The enzyme, pyranose dehydrogenase (PDH), from the filamentous fungus Coprinopsis cinerea (CcPDH) of the Basidiomycete division, is composed of a catalytic PQQ-dependent domain classified as a member of the novel auxiliary activity family 12 (AA12), an AA8 cytochrome b domain, and a family 1 carbohydrate-binding module (CBM1), as defined by the Carbohydrate-Active Enzymes (CAZy) database. In the catalytic cycle of CcPDH, electrons are transferred from the reduced PQQ in the AA12 domain to heme b in the AA8 domain, which acts as a built-in mediator and transfers electrons to a heterogeneous electron acceptor. Therefore, CcPDH is thought to be involved in the extracellular oxidative degradation of the plant cell wall. Here, we present the crystal structures of the AA12 domain in its apo- and holo-forms and the AA8 domain of this enzyme.

The AA8 domain of CcPDH was determined at a 1.8-Å resolution, and the final model was refined to R and Rfree values of 15.7% and 20.4%, respectively. The asymmetric unit of the AA8 domain crystal contains a single AA8 domain (residues 21 to 215 of the full-length CcPDH) with a single b-type heme, 2 2-methyl-2,4-pentanediol molecules, 1 acetate ion, and 155 water molecules. AA8 proteins fold into an immunoglobulin-like β-sandwich with a Met/His-coordinated b-type heme. One disulfide bond (Cys138-Cys141) that is conserved in the AA8 domain of CDHs from various filamentous fungi was observed. Asn140 is glycosylated with a single GlcNAc molecule, as predicted by the NetNGlyc (version 1.0) server. The heme iron is hexacoordinated with Met83 and His182, which serve as axial ligands, and coordination distances of approximately 2.4 Å and 2.0 Å are observed between the heme iron and the S-γ atom of Met83 and the N-σ2 atom of His182, respectively. The main-chain coordinates of the AA8 domain of CcPDH closely resemble those of the AA8 domain of PcCDH, whereas the amino acid residues surrounding the heme are different. On the other hand, Tyr108 in CcPDH is conserved in CDHs and forms a hydrogen bond with the d-propionate side chain of the heme b. Interestingly, Glu162 in PcCDH corresponds to Arg181 in CcPDH, which interacts with the propionate group of the heme, which results in a local positive charge at the heme binding pocket of the AA8 domain. The crystal structure analysis of the AA8 domain of CcPDH revealed that Arg181 is located in the heme binding pocket and interacts with a propionate group of the heme, making the local surface positively charged around the heme, while most AA8 domains from basidiomycetous CDHs have a Glu residue at the corresponding position, and CcPDH is the only family member with an Arg at that position.

> QGSPTQWYDSITGVTFSRFYQQDTDASWGYIFPSASGGQAPDEFIGLFQGPASAGWIGNSLGGSMRNNPLLVGWVDGSTPRISARWATDYAPPSIYSGPRLTILGSSGTNGNIQRIVYRCQNCTRWTGGAGGIPTTGSAVFGWAFHSTTKPLTPSDPSSGLYRHSHAAQYGFDIGNARTTLYDYYLQQLTNAPPLSG> MSLSAQADARPTPAPSFSGVTVDGKPFSSASLKGKAYIVNFFATWCPPCRSEIPDMVQVQKTWASRGFTFVGIAVNEQLPNVKNYMKTQGII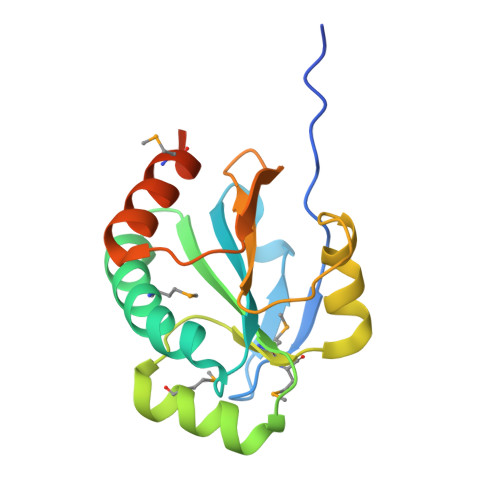YPVMMATPELIRAFNGYIDGGITGIPTSFVIDASGNVSGVIVGPRSKADFDRIVKMALGAKAATKEGHHHHHH>[2x]GPLGSGGLFFNALKNDKENFTVLQTIRQQQSTLNGSWVALLQTRNTLNRAGIRYMMDQNNIGSGSTVAELMESASISLKQAEKNWADYEA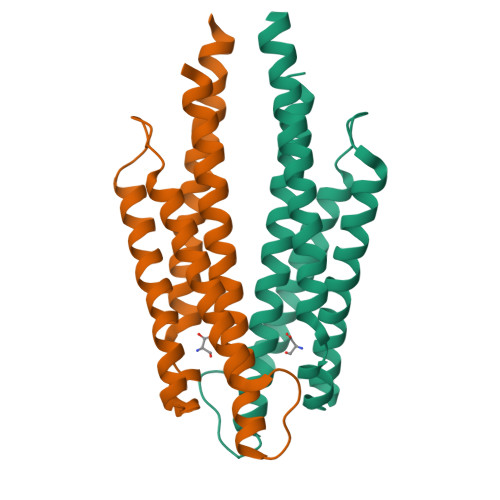LPRDPRQSTAAAAEIKRNYDIYHNALAELIQLLGAGKINEFFDQPTQGYQDGFEKQYVAYMEQNDRLHDIAVSDNNASYS~{N}-[2-(4-fluorophenyl)ethyl]furan-2-carboxamide | C13 H12 F N O2 | 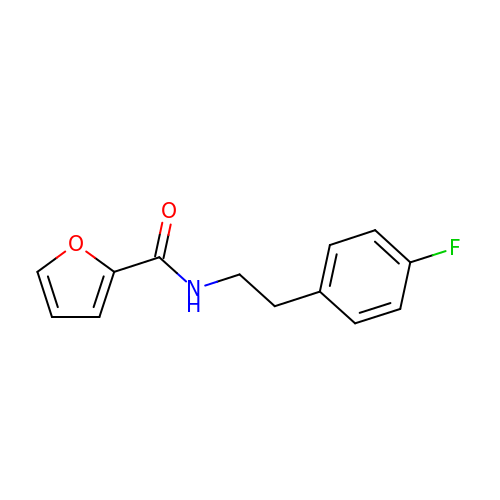GSMVTQDRELNXRQ-UHFFFAOYSA-N> RGKVKWFHDYYGYGFITKDEGGDVFVNADAIDMEGFKTLKEGQVVEFE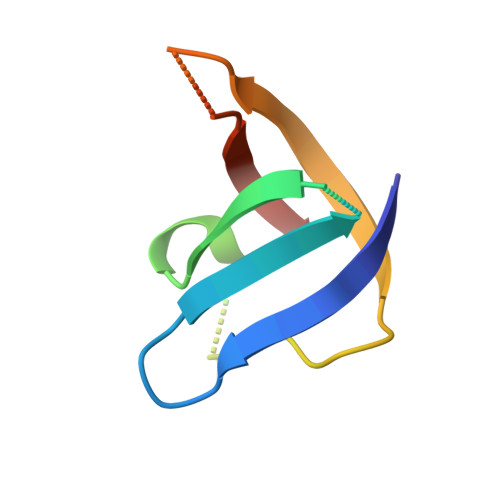IDSTVANAPQAAHVKVVE>[3x]MSVEDTQPLITHLIELRKRLLNCIIAVIVIFLCLVYFANDIYHLVSAPLIKQLPQGSTMIATDVASPFFTPIKLTFMVSLILSAPVILYQVWAFIAPALYKHERRLVVPLLVSSSLLFYIGMAFAYFVVFPLAFGFLANTAPEGVQVSTDIASYLSFVMALFMAFGVSFEVPVAIVLLCWMGITSPEDLRKKRPYVLVGAFVVGMLLTPPDVF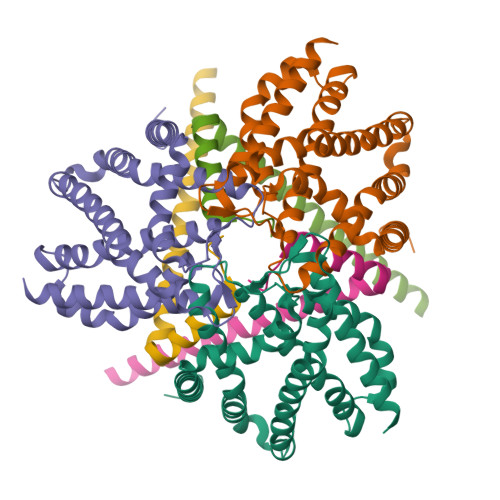SQTLLAIPMYCLFEIGVFFSRFYVGKGRNREEENDAEAESEKTEERSHHHHHH;>MFDIGFSELLLVFIIGLVVLGPQRLPVAVKTVAGWIRALRSLATTVQNELTQELKLQEFQDSLKKVEKASLTNLTPELKASMDELRQAAESMKRSYVANDPEKASDEAHTIHNPVVKDNEAAHEGVTPAAAQTQASSPEQKPETTPEPVVKPAADAEPKTAAPSPSSSDKP[3x]(~{E})-3-(1,3-benzodioxol-5-yl)-1-(3-nitrophenyl)prop-2-en-1-one 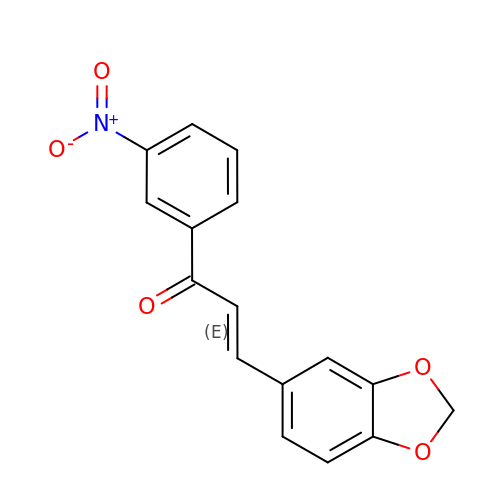| C16 H11 N O5 | MALGARLLWBWYQV-GQCTYLIASA-N> GPHMLEVPPQPQYSYHDINVYSLAGLAPHITLNPTIPLFQAHPQLKQCVRQAIERAVQELVHPVVDRSIKIAMTTCEQIVRKDFALDSEESRMRIAAHHMMRNLTAGMAMITCREPLLMSISTNLKNSFAS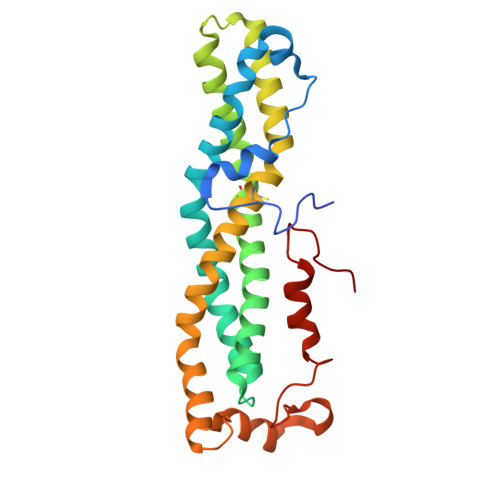ALRTASPQQREMMDQAAAQLAQDNCELACCFIQKTAVEKAGPEMDKRLATEFELRKHARQEGRRYCDPVVLTYQAERMPEQIRLKVGGVDPKQLAVYEEFARNVPGFLPTNDL>[3x]MFYINSKYKIDLDKIMTKMKNKSVINIDDVDDEELLAILYTSKQFEKILKNNEDSKYLENKVFCSVFLEPSTRTRCSFDAAILKLGSKVLNITDMNSTSFYKGETVEDAFKILSTYV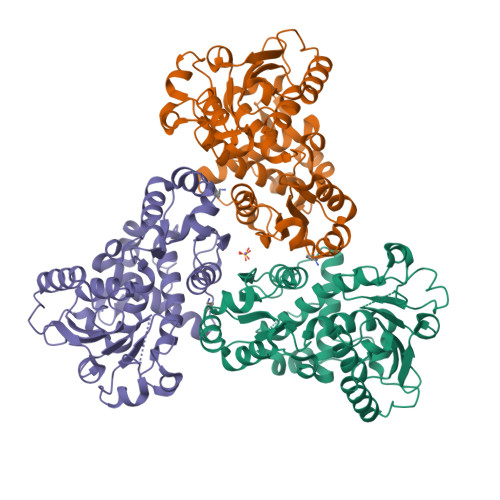DGIIYRDPSKKNVDIAVSSSSKPIINAGNGTGEHPTQSLLDFYTIHNYFPFILDRNINKKLNIAFVGDLKNGRTVHSLSKLLSRYNVSFNFVSCKSLNIPKDIVNTITYNLKKNNFYSDDSIKYFDNLEEGLEDVHIIYMTRIQKERFTDVDEYNQYKNAFILSNKTLENTRDDTKILHPLPRVNEIKVEVDSNPKSVYFTQAENGLYVRMALLYLIFSSTSSAWSHPQFEK>[2x]MPAPHGLSPLSKAFLMRRAFQRRILPHSLAMALSLPLAGYVQAQEVEFDIPPQALGSALQEFGRQADIQVLYRPEEVRNKRSSAIKGKLEPNQAITELLRGTGASVDFQGNAITISVAEAADSSVDLGATMITSNQLGTITEDSGSYTPGTIATATRLVLTPRETPQSITVVTRQNMDDFGLNNIDDVMRHTPGITVSAYDTDRNNYYARGFSINNFQYDGIPSTARNVGYSAGNTLSDMAIYDRVEVLKGATGLLTGAGSLGATINLIRKKPTHEFKGHVELGAGSWDNYRSELDVSGPLTESGNVRGRAVAAYQDKHSFMDHYERKTSVYYGILEFDLNPDTMLTVGADYQDNDPKGSGWSGSFPLFDSQGNRNDVSRSFNNGAKWSSWEQYTRTVFANLEHNFANGWVGKVQLDHKINGYHAPLGAIMGDWPAPDNSAKIVAQKYTGETKSNSLDIYLTGPFQFLGREHELVVGTSASFSHWEGKSYWNLRNYDNTTDDFINWDGDIGKPDWGTPSQYIDDKTRQLGSYMTARFNVTDDLNLFLGGRVVDYRVTGLNPTIRESGRFIPYVGA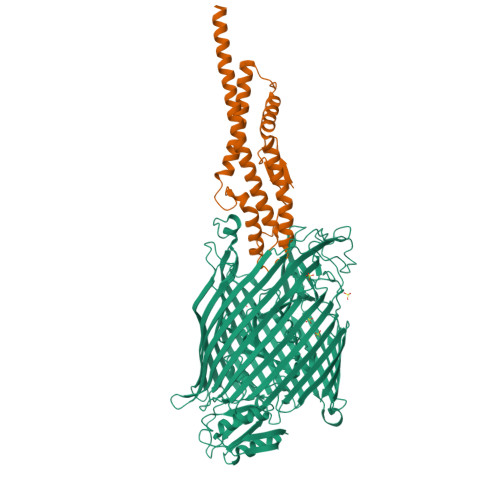VYDLNDTYSVYASYTDIFMPQDSWYRDSSNKLLEPDEGQNYEIGIKGEYLDGRLNTSLAYFEIHEENRAEEDALYNSKPTNPAITYAYKGIKAKTKGYEAEISGELAPGWQVQAGYTHKIIRDDSGKKVSTWEPQDQLSLYTSYKFKGALDKLTVGGGARWQGKSWQMVYNNPRSRWEKFSQEDYWLVDLMARYQITDKLSASVNVNNVFDKTYYTNIGFYTSASYGDPRNLMFSTRWDF;>[2x]MAVNDYEPGSMVITHVQGGGRDIIQYIPARSSYGTPPFVPPGPSPYVGTGMQEYRKLRSTLDKSHSELKKNLKNETLKEVDELKSEAGLPGKAVSANDIRDEKSIVDALMDAKAKSLKAIEDRPANLYTASDFPQKSESMYQSQLLASRKFYGEFLDRHMSELAKAYSADIYKAQIAILKQTSQELENKARSLEAEAQRAAAEVEADYKLEHHHHHH> MEDISEPPLHDFYCSRLLDLVFLLDGSSRLSEAEFEVLKAFVVDMMERLRISQKWVRVAVVEYHDGSHAYIGLKDRKRPSELRRIASQVKYAGSQVASTSEVLKYTLFQIFSKIDRPEASRIALLLMASQEPQRMSRNFVRYVQGLKKKKVIVIPVGIGPHANLKQIRLIEKQAPENKAFVLSSVDELEQQRDEIVSYLCDLAPEAPPPTLPPH;> HPIC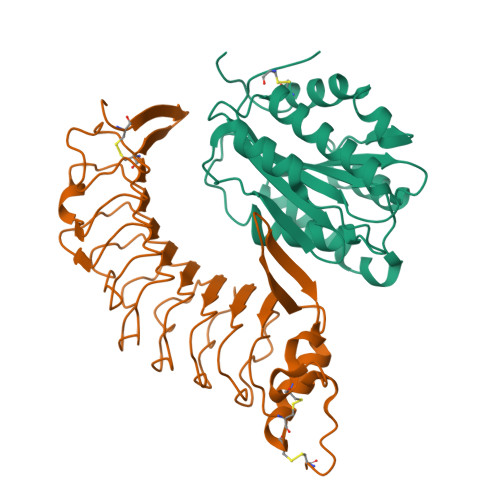EVSKVASHLEVNCDKRDLTALPPDLPKDTTILHLSENLLYTFSLATLMPYTRLTQLNLDRCELTKLQVDGTLPVLGTLDLSHNQLQSLPLLGQTLPALTVLDVSFNRLTSLPLGALRGLGELQELYLKGNELKTLPPGLLTPTPKLEKLSLANNDLTELPAGLLNGLENLDTLLLQENSLYTIPKGFFGSHLLPFAFLHGNPWLCNCEILYFRRWLQDNAENVYVWKQGVDVKAMTSNVASVQCDNSDKFPVYKYPGKGCPTLGDEGDTDLYDYYPEEDTEGDK>[2x]MQVSRRALLAGISGASLTAAFPMPVLAAVNQASDDYRDRSLSPARRAAALANLMTLDEMAAQLNCPRAADVMSDPAGFEADFPYFAHGIGGVYSASLEAGPEDNARAVMAMQQEVVSRSRFGIPAFVFEECLHGLLADGATQFPQAMAMACAFRPDMVRQVFEATAKEARSRGSQGCFSPNIDICTDPRWGRSEETWGEDPHVVTVSAKAIVEGLQGAPAEYLPANRIATSVKHFAGYGQGIGGRNFAPSHIGPVEMQNVVLPPFRAAITEAGSIGLMASHGEIDGVPAHADTHLLNDVLRDDWGFEGYVVSDWDDVRRIHSLHGVAGSEAEAAIMGLRAGVDIELANNGVYLMLPQLVRDGLLEERYVRRAAERILAAKFKCGLFDMPFADPALAGRLARSTEHKLLARRMAEESIVLLQNEGNVLPLQSSAVRKMLVVGPNAASVHLGGYSPKPFVGVSALEGLQAYAEQAGFEVE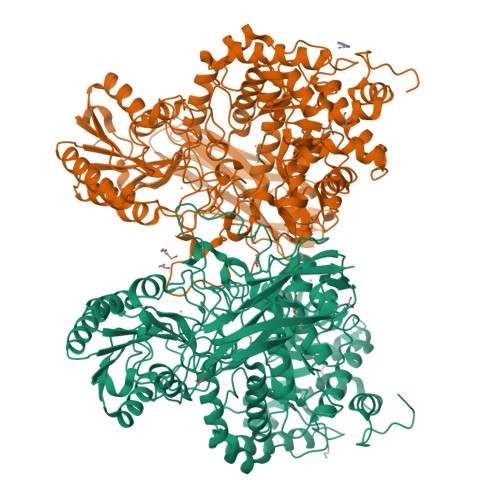YAQGCAITAGDEGNNEIETDASDESVQADPARNRRLIAEAVATAQDCDVIVMCLGGNESTAREAYFAGDSRGDRDDLELIGEQNELAEALLALGKTTVAVLIHGRPLSPLVLAENCPAILDAFYPGEQGGHAIASILFGDVNPSGKLPVTIVRNVGQLPGYYYQKPTGRFRNYVFSDSTPLYPFGHGLSYTSFGYGAPQAERASIGLQDRLRVSVSVRNTGDRAGQDVVQLYIRDSIASRARPIKEMRGFQKVLLEPGEVQVVQFELGPEDFGYRDADGKLLVEPGEIVIMAGPDSQNLQETRITLV CISs are macromolecular injection devices with an overall structure that is homologous to the contractile tails of bacteriophages. Their conserved modules include an inner tube, a contractile sheath and a baseplate complex. For firing of the extended apparatus, the baseplate undergoes a conformational change and triggers sheath contraction, which in turn causes the inner tube to be expelled and injected into a target. Here we performed structural and mechanistic studies on a clade Ib CIS gene cluster in the marine bacterium Algoriphagus machipongonensis PR1.

The distal AlgoCIS end is terminated by a hexameric cap complex of Alg16A, and – in contrast to other known eCISs – a hexameric complex of Alg16B, hereafter referred to as the ‘cap adaptor’. The dome-shaped Alg16A cap complex covers the inner tube, and it exhibits an ~11-Å-wide central channel. Each Alg16A subunit interacts with three Alg1 proteins from the distal inner tube layer (Alg1-L22) and terminates the tube. Compared with homologues in PVC/AFP, Alg16A is much shorter (197 amino acids in Alg16A, 293 in Pvc16, 295 in Afp16) and folds into a single domain with a C-terminal extension. Interestingly, the cap adaptor Alg16B mediates the interactions between the cap complex Alg16A and the most distal sheath layer (Alg2-L23). The cap adaptor expands the outer diameter of the cap to ~164 Å, with an enlarged inner diameter of ~115 Å. The Alg16B NTD (residues 1–213) is an immunoglobulin-like domain flanked by three additional α-helices (α1–3), whereas one single β-barrel constitutes a C-terminal domain (CTD) (residues 214–284). The Alg16B adopts a parallel arrangement with Alg16A. The N terminus of Alg16B interacts with the C terminus of Alg16A in a mimicked ‘handshake’ manner, terminating the sheath assembly. Moreover, the tube lumen was empty for all observed particles in AlgoCIS ΔAlg16B. Together, these results showed that the cap adaptor plays an important role in stabilizing the cap module and the most distal sheath layer, and its absence results in mis-assembled particles.

>MIFEVLKILTDEVNQNFKGLEMEDSEVVLNNVALIDSQQDVATELQNKVILSMINLREEVTMKNFPNNVLEGTKVTYKNPKLNINLFLIFCANRTGYKKSLSDLSRILEFFQHKSVFTQSNTSFDRDLEEMENVKNFRFTMELFTPTFEELNYIWGTLGGRQYPSVFYKLNLIVIDRDATTSEEGVITNIHRNYETL[6x];>[6x]MQVSSSFRSFLKLDILHSYFLNDGEKDFSSMNEEESKTQLKSYNWKDFLEIYPSQKTSHMMRGNKIFFKSFNDSIILAIKVESGTENQPFNELYEDESMTFLLSLKDQYFGNYTDLDLADQLLYFSNKTPVLPEAFTFKPIDRINQSGTVGEEYLYEGENKKHLLEEAHLNPGGGVLGIIQIYMKGDTPVLSLINNDGTLKNSLPHFKIHFSNRKSTWKYINLKDDFETETKKDYPLTKFGFILLDKKSDFISPPAHFEKYVFPNPDARRIKITPTKNYSEIFI;>MSYPLSKFHFSVEWGGTKIGFTEVSGLDLETEIIEYRHGASPEYSKIKMPGMQKFSNITLKRGTFKSDNEYFQWYNTINLNKVERRDLTISLLNEEHEPVVTWKVKNAWPLKVQSTDLKGDGNEVAIESMELAHEGLVIQNE[12x];>[6x]MATYKTPGVYIEEITKFPPSVAQVETAIPAFIGYTQFARTKPSVDSDDLILKPKRISSLLDFTTYYGGAQNEQGITVKLTDTLIEGAENRTINVPEPTFKSPYLMFYSLQMYFANGGGPCYIVSTGVYDDWSDSETPPTINFSDLESGLAVIRKEDEPTLLLFPDATNLPTDDEFYSLYNSALMQCNDLQDRFTILDTYSDQTYNDGVEDLDPIPALRNGINLTKDYLKYGAAYYPFVQTILNYQYSADEIVIQHLSYNPNAIATALDNLNAVNGPTFIDAILDDLRDLSLPDISGEISDAVGFMYDDVDGFDIDGTFTTNSVKVANFASLVESVLSTLNELIDAKEEINKDVNSAIASSEEDNAIKTAISDALDVFNEDFEGADKIESVAKNLSDLLIKIKQADTNTKVENVLSINALNFSAEFEKLLTYDVNTGLTASVTLDLFANIGTRLDDIIAAVSAAEPIDVNNGKLNGRLLSDIEPLDNATYNTILLEINSHKVTLPPSSSMAGAYARVDNDRGVWKSPANIGLNYVSKPSVTVSHEEQESMNVHGTGKSVNAIRSFVGKGTLVWGARTLAGNDNEWRYISVRRFFNMAEESIKKATEQFVFEPNDGNTWVRVRAMIENFLILQWRAGALAGAKPEHAFYVKVGLGQTMTAQDILEGNMNVEIGLAVVRPAEFIILKFSHKMQES> MAMRQCAIYGKGGIGKSTTTQNLVAALAEMGKKVMIVGCDPKADSTRLILHSKAQNTIMEMAAEAGTVEDLELED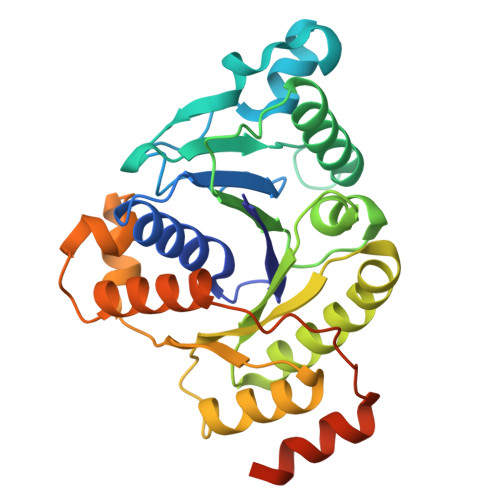VLKAGYGGVKCVESGGPEPGVGCAGRGVITAINFLEEEGAYEDDLDFVFYDVLGDVVCGGFAMPIRENKAQEIYIVCSGEMMAMYAANNISKGIVKYANSGSVRLGGLICNSRNTDREDELIIALANKLGTQMIHFVPRDNVVQRAEIRRMTVIEYDPKAKQADEYRALARKVVDNKLLVIPNPITMDELEELLMEFGIMEVEDESIVGKTAEEV>[2x]MSTQYETQGYTINNAGRRLVVDPITRIEGHMRCEVNINDQNVITNAVSCGTMFRGLEIILQGRDPRDAWAFVERICGVCTGVHALASVYAIEDAIGIKVPDNANIIRNIMLATLWCHDHLVHFYQLAGMDWIDVLDALKADPRKTSELAQSLSSWPKSSPGYFFDVQNRLKKFVEGGQLGIFRNGYWGHPQYKLPPEANLMGFAHYLEALDFQREIVKIHAVFGGKNPHPNWIVGGMPCAINIDESGAVGAVNMERLNLVQSIITRTADFINNVMIPDALAIGQFNKPWSEIGTGLSDKCVLSYGAFPDIANDFGE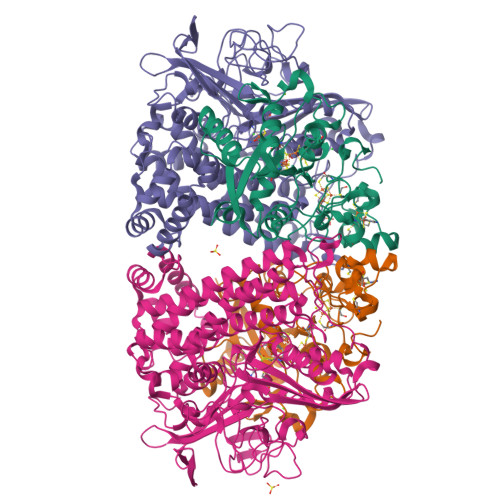KSLLMPGGAVINGDFNNVLPVDLVDPQQVQEFVDHAWYRYPNDQVGRHPFDGITDPWYNPGDVKGSDTNIQQLNEQERYSWIKAPRWRGNAMEVGPLARTLIAYHKGDAATVESVDRMMSALNLPLSGIQSTLGRILCRAHEAQWAAGKLQYFFDKLMTNLKNGNLATASTEKWEPATWPTECRGVGFTEAARGALGHWAAIRDGKIDLYQCVVPTTWNASPRDPKGQIGAYEAALMNTKMAIPEQPLEILRTLHSFDPCLACSTH;>LENKPRIPVVWIHGLECTCCTESFIRSAHPLAKDVILSLISLDYDDTLMAAAGTQAEEVFEDIITQYNGKYILAVEGNPPLGEQGMFCISSGRPFIEKLKRAAAGASAIIAWGTCASWGCVQAARPNPTQATPIDKVITDKPIIKVPGCPPIPDVMSAIITYMVTFDRLPDVDRMGRPLMFYGQRIHDKCYRRAHFDAGEFVQSWDDDAARKGYCLYKMGCKGPTTYNACSSTRWNDGVSFPIQSGHGCLGCAENGFWDRGSFYSRVVDIPQMGTHSTADTVGLTALGVVAAAVGVHAVASAVDQRRRHNQQPTETEHQPGNEDKQARSHHHHHH[2x]>MKYILVTGGVISGIGKGIIASSIGTILKSCGLRVTAIKIDPYINIDAGTFSPYEHGEVFVLNDGGEVDLDLGNYERFLDINLYKDNNITTGKIYQHVINKERRGDYLGKTVQVVPHITDAVQEWVMNQAKVPVDGNKEEPQICVIELGGTIGDIEGMPFVEAFRQFQFKAKRENFCNIHVSLVPQLSATGEQKTKPTQNSVRALRGLGLSPDLIVCRSSTPIEMAVKEKISMFCHVNPEQVICIHDVSSTYRVPVLLEEQSIVKYFKERL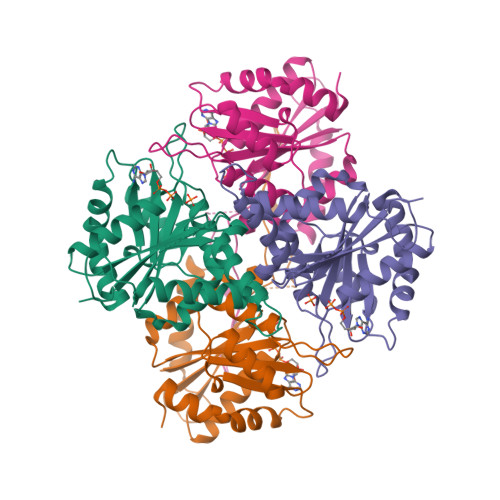HLPIGAHHHHHH[2x]>[6x]GPLGSMRLHDFVSKTVIKPESCVPCGKRIKFGKLSLKCRDCRVVSH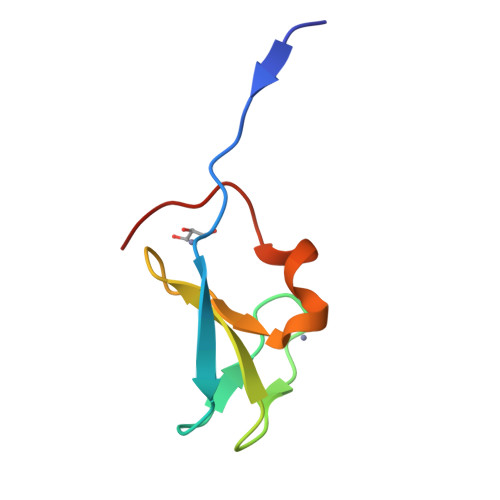PECRDRCPLPCIPTL> MDVIPLSLGLETMGGLVEKVIPRNTTIPVARAQDFTTFKDGQTAMSIHVMQGERELVQDCRSLARFALRGIPALPAGGAHIRVTFQVDADGLLSVTAMEKSTGVEASIQVKPSYGLTDSEIASMIKDSMSYAEQDVKARMLAEQKVEAARVLESLHGALAADAALLSAAERQVIDDAAAHLS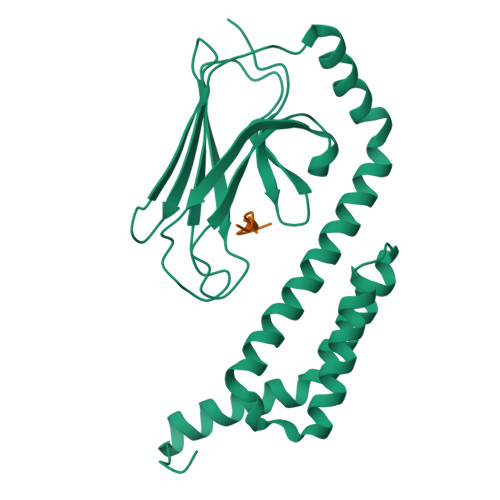EVAQGDDVDAIEQAIKNVDKQTQDFAARRMDQSVRRALKGHSVDE;> ELPPVKIHC> MERQQQQQQQLRNLRDFL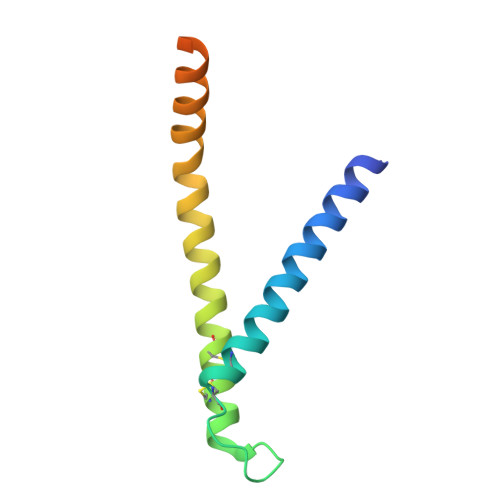LVYNRMTELCFQRCVPSLHHRALDAEEEACLHSCAGKLIHSNHRLMAAYVQLMPALVQRRIADYEAASAVPGVAAEQPGVSPSGS> LTNSSLMPTLNPMIQQLALAIAASWQSLPLKPYQLPEDL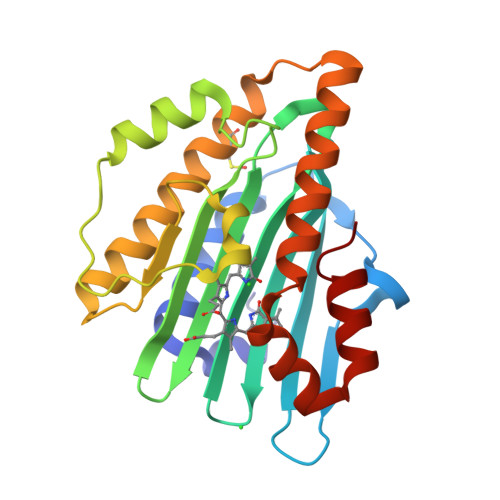GYVEGRLEGEKLVIENRCYQTPQFRKMQLELAKVGKGLDILHCVMFPEPLYGLPLFGCDIVAGPGGVSAAIADLSPTQSDRQLPAAYQKSLAELGQPEFEQQRELPPWGEIFSEYCLFIRPSNVTEEERFVQRVVDFLQIHCHQSIVAEPLSEAQTLEHRQGQIHYCQQQQKNDKTRRVLEKAFGEAWAERYMSQVLFDV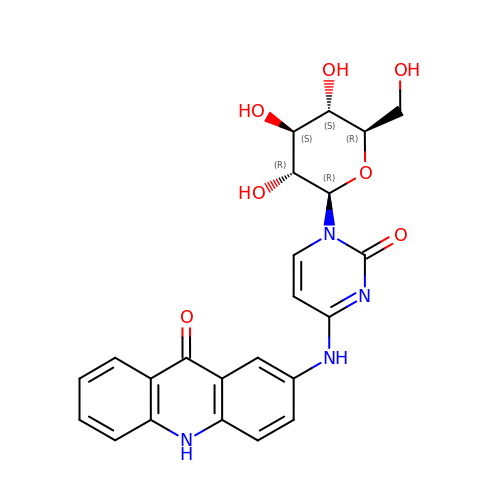2-[[1-[(2~{R},3~{R},4~{S},5~{S},6~{R})-6-(hydroxymethyl)-3,4,5-tris(oxidanyl)oxan-2-yl]-2-oxidanylidene-pyrimidin-4-yl]amino]-10~{H}-acridin-9-one | C23 H22 N4 O7 | GFASNZAXNSUSSV-RECXWPGBSA-N> MSMLKREDWYDLTRTTNWTPKYVTENELFPEEMSGARGISMEAWEKYDEPYKITYPEYVSIQREKDSGAYSIKAALERDGFVDRADPGWVSTMQLHFGAIALEEYAASTAEARMARFAKAPGNRNMATFGMMDENRHGQIQLYFPYANVKRSRKWDWAHKAIHTNEWAAIAARSFWDDMMMTRDSVAVSIMLTFAFETGFSNMQFLGLAADAAEAGDHTFASLISSIQTDESRHAQQGGPSLKILVENGKKDEAQQMVDVAIWRSWKLFSVLTGPIMDYYTPLESRNQSFKEFMLEWIVAQFERQLLDLGLDKPWYWDQFMQDLDETHHGMHLGVWYWRPTVWWDPAAGVSPEEREWLEEKYPGWNDTWGQCWDVITDNLVNGKPELTVPETLPTICNMCNLPIAHTPGNKWNVKDYQLEYEGRLYHFGSEADRWCFQIDPERYKNHTNLVDRFLKGEIQPADLAGALMYMSLEPGVMGDDAHDYEWVKAYQKKTNAA;> MSEQQPEALKPLKTWSHLAGNRRRPSEYEVVSTNLHYFTDNPERPWELDSNLPMQTWYKKYCFDSPLKHDDWNAFRDPDQLVYRTYNLLQDGQESYVQGLFDQLNDRGHDQMLTREWVETLARFYTPARYLFHALQMGSVYIHQIAPASTITNCATYETADHLRWLTHTAYRTRELANCYPDVGFGKRERDVWENDPAWQGFRELIEKALIAWDWGEAFTAINLVTKPAVEEALLQQLGSLAQSEGDTLLGLLAQAQKRDAERHRRWSSALVKMALEKEGNREVLQKWVAKWEPLAD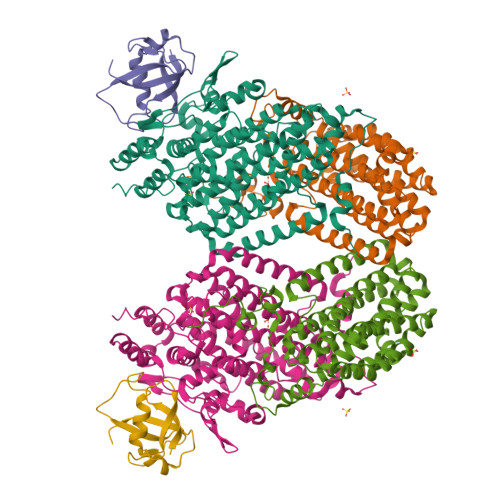KAIEAYCSALPDGENAIVEAKSASRYVRQMMGL;> MATFPIMSNFERDFVIQLVPVDTEDTMDQVAEKCAYHSINRRVHPQPEKILRVRRHEDGTLFPRGMIVSDAGLRPTETLDIIFMDN> TYVQHIKRRDIVLKRELGEGAFGKVFLAECYNLSPTKDKMLVAVKALKDPTLAARKDFQREAELLTNLQHEHIVKFYGVCGDGDPLIMVFEYMKHGDLNKFLRAHGPDAMILVDGQPRQAKGELGLSQMLHIASQIASGMVYLASQHFVHRDLATRNCLVGANLLVKIGDFGMSRDVYSTDYYRLFNPSGNDFCIW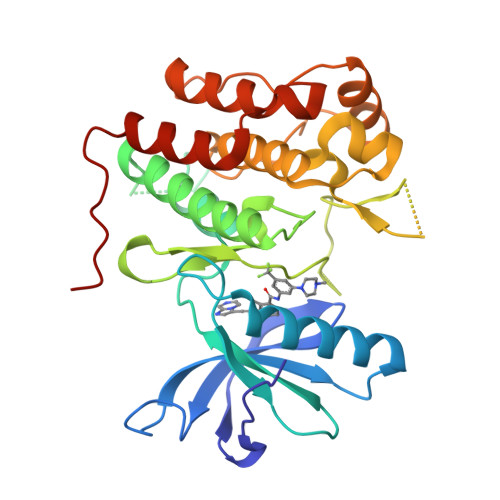CEVGGHTMLPIRWMPPESIMYRKFTTESDVWSFGVILWEIFTYGKQPWFQLSNTEVIECITQGRVLERPRVCPKEVYDVMLGCWQREPQQRLNIKEIYKILHALGKATPIYLDILG>[2x]SLRANDAPIVLLHGFTGWGREEMFGFKYWGGVRGDIEQWLNDNGYRTYTLAVGPLSSNWDRACEAYAQLVGGTVDYGAAHAAKHGHARFGRTYPGLLPELKRGGRIHIIAHSQGGQTARMLVSLLENGSQEEREYAKAHNVSLSPLFEGGHHFVLSVTTIATPHDGTTLVNMVDFTDRFFDLQKAVLEAAAVASNVPYTSQVYDFKLDQWGLRRQPGESFDHYFERL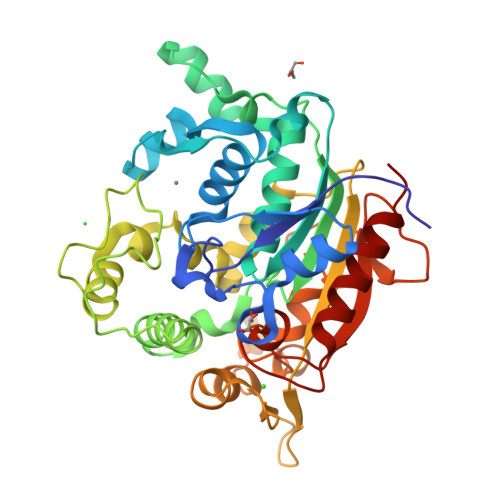KRSPVWTSTDTARYDLSVSGAEKLNQWVQASPNTYYLSFSTERTYRGALTGNHYPELGMNAFSAVVCAPFLGSYRNPTLGIDERWLENDGIVNTVSMNGPKRGSSDRIVPYDGTLKKGVWNDMGTYNVDHLEIIGVDPNPSFDIRAFYLRLAEQLASLQP> KKDGYPVEYDNCAYICWNYDNAYCDKLCKDKKADSGYCYWVHILCYCYGLPDSEPTKTNGK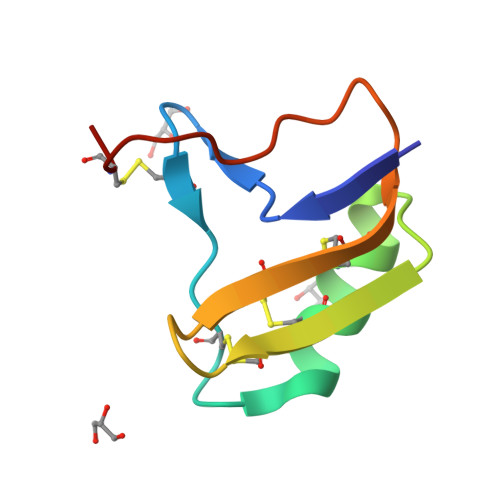CKS>SVAADSAATESLGRIGSLSQVSGVLGCQWGDEGKGKLVDILAQHFDIVARCQGGANAGHTIYNSEGKKFALHLVPSGILNEDTTCVIGNGVVVHLPGLFKEIDGLESNGVSCKGRILVSDRAHLLFDFHQEVDGLRESELAKSFIGTTKRGIGPAYSSKVIRNGIRVGDLRHMDTLPQKLDLLLSDAAARFQGFKYTPEMLREEVEAYKRYADRLEPYITDTVHFINDSISQKKKVLVEGGQATMLDIDFGTYPFVTSSSPSAGGICTGLGIAPSVVGDLIGVVKAYTTR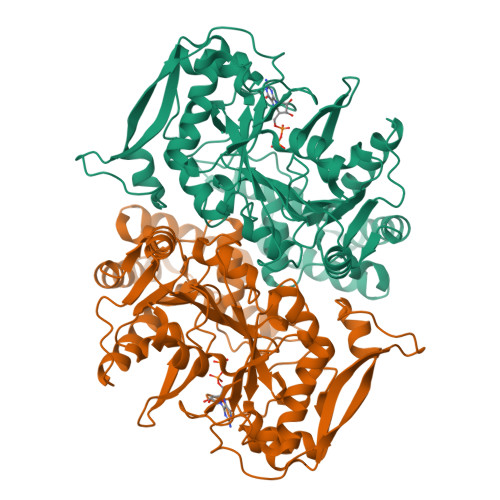VGSGPFPTENLGTGGDLLRLAGQEFGTTTGRPRRCGWLDIVALKFSCQINGFASLNLTKLDVLSDLNEIQLGVAYKRSDGTPVKSFPGDLRLLEELHVEYEVLPGWKSDISSVRNYSDLPKAAQQYVERIEELVGVPIHYIGIGPGRDALIYK[2x]>[2x]MYRKGAQAERELIKLLEKHGFAVVRSAGSKKVDLVAGNGKKYLCIEVKVTKKD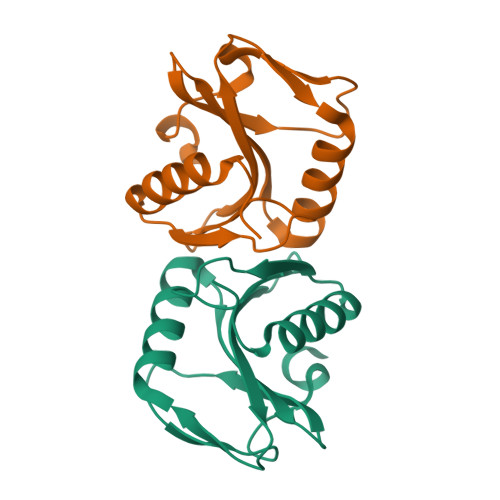HLYVGKRDMGRLIEFSRRFGGIPVLAVKFLNVGWRFIEVSPKIEKFVFTPSSGVSLEVLLGIQKTLEGKS> SGKGKGKRTHFNQFAYDGNTYDLEVPVLLVPEDKSQKPYVAIIKDITQTKDGSMMILGQWFYRPEEAEKRGGGNWQSSDTRELFYSFHRDEVPAESVMHRCVVYFVPAHKQLPKRKNNPGFIVRKVYDTVEKKLWKLTDKDYEDSKQREIDVLVKKTMNVLGDLPDLES;> LATKAA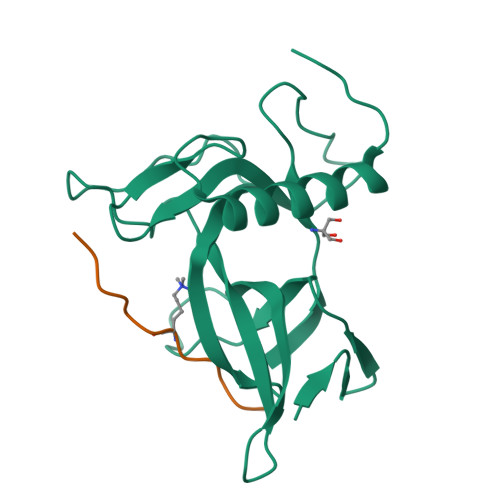RKSAPATGGVKK> MQKTLEVWIMPNSPQPAEDFKALVAPFEKAHGVEVKVTVLDWGVAWTKITTAATSGVGPDLTQLGTTWVGAISAMGVLEPVDDVLEALGGEKAYLPAVWRTTRLEGARQATAVPWFSELRAFYYRTDALKAAGVNPAEMFASWQGFEAGLARLKASSFRDPETKAPLAPLCTPGRTPRTLHNAAPWIWGAGGEIVRQAGGRWQSALNSPESLEGLYFFLSLAQKGYVPAESLEKNTAQIEADFQAGKCAVFASGPWMIQRAQVPEAKGGFAERTAAKNLGVAPYPAGPKGRYTFFGGSNLALFNFSKNKPLAKELLKYLGGPEAQVRYAQMTGMLPALRSAWSDPSFQQN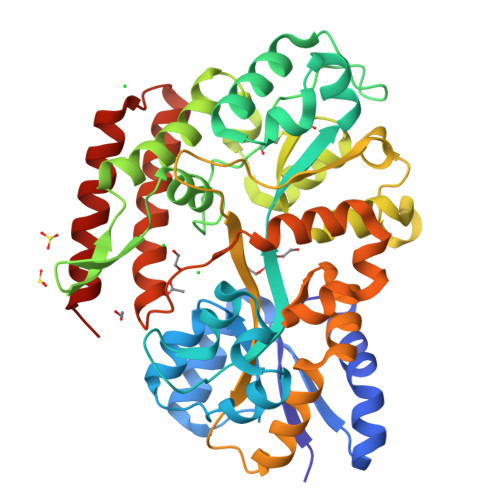PLLRTFIQAAQFGRTYPSLAGWGGVENLAVQHLGMAWDLVAQGRLTREALKDLMDKASAAINQALRHHHHHH> TEPISHMQEKPATLRLRGLPYRTTAEDIANFFEGYSLAGPPDE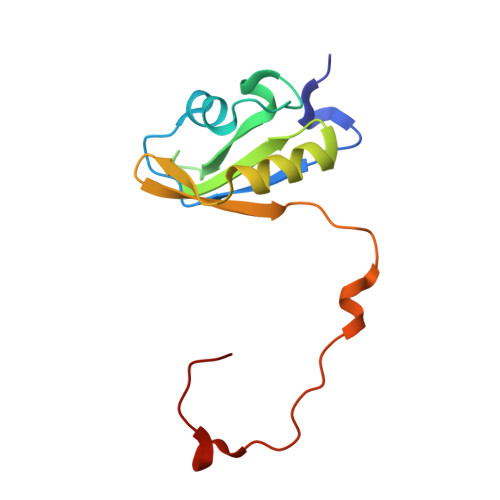AIQLHRRMDGRPTGWASVYFESEQEARRAKQDKHRSYLHGRYIEIFINFETGELEWIHQPQLSENVNRKHHGKDNRG> GSGPPGPPGPPGPPGAR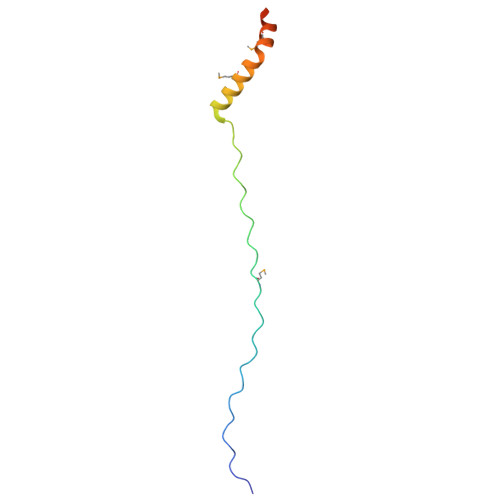GQAGVMGFPGPPGPPGPPGRAPTDQHIKQVCMRVIQEHFAEMAASLKRPDSGAT> IIGGTECKPHSRPYMAYLEIVTSNGPSKFCGGFLIRRNFVLTAAHCAGRSITVTLGAHNITEEEDTWQKLEVIKQFRHPKYNTSTLHHDIMLLKLKEKASLTLAVGTLPFPSQKNFVP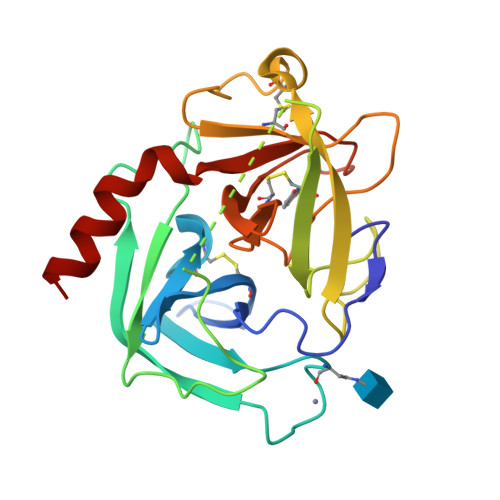PGRMCRVAGWGRTGVLKPGSDTLQEVKLRLMDPQACSHFRDFDHNLQLCVGNPRKTKSAFKGDSGGPLLCAGAAQGIVSYGRSDAKPPAVFTRISHYQPWINQILQAN> E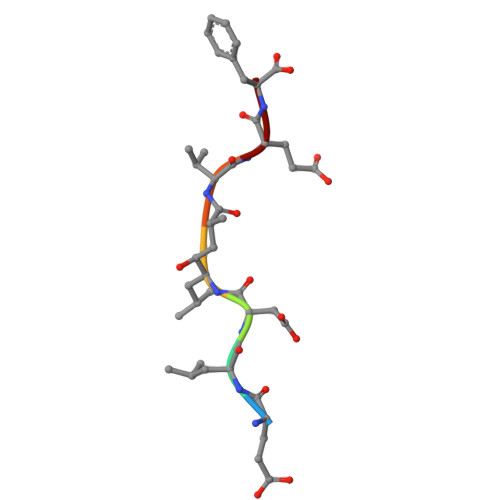LDXVEF>[4x]MAHHHHHHMLTRFLIQEQHAGRINADLRQLIAVVARACTSISIAVSKGALGGVLGDAGTGNVQGEAQKKLDV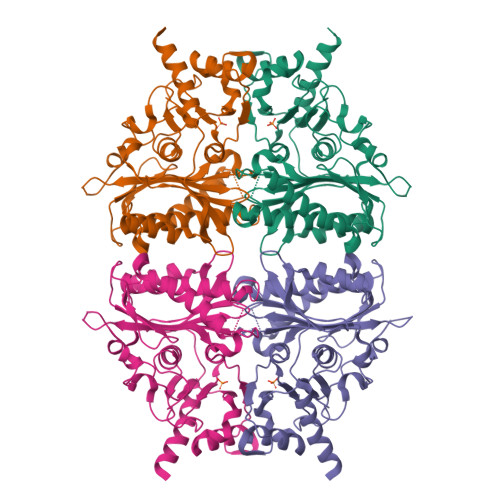ISNEILLEANAWGGHLAACASEEMDHSQPVPDIYPRGDFLLLFDPLDGSSNIDVNVSVGTIFSVLRCPTNVELPGDDAFLQPGSKQIAAGYCIYGPSTQLVLTVGHGTHAFTLDREKGEFVLTTENMQIPAATQEFAINMSNQRHWEAPMQAYVGDLLAGKEGTRGKNFNMRWIASMVADVHRILTRGGIFIYPWDKKDPSKAGKLRLMYEANPMGLLVEQAGGAAWTGRERILDIQPDQLHQRVPVFLGSREEVAEAVRYHHAHDNAQG(2S)-2-[(2,1,3-BENZOTHIADIAZOL-4-YLSULFONYL)AMINO]-2-PHENYL-N-PYRIDIN-4-YLACETAMIDE | C19 H15 N5 O3 S2 | 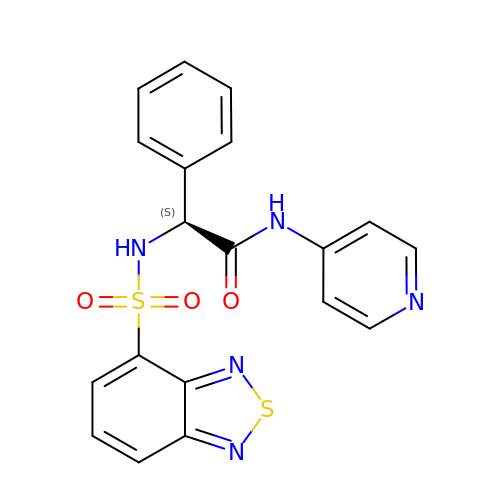ADRNPUSZBRQDBG-KRWDZBQOSA-N> GKAFDDGAFTGIREINLSYNKETAIGDFQVVYDLNGSPYVGENHKSFITGFTPVKISLDFPSEYIMEVSGYTGKVSGYVVVRSLTFKTNKKTYGPYGVTSGTPFSLPIENGLIVGFKGSIGYWL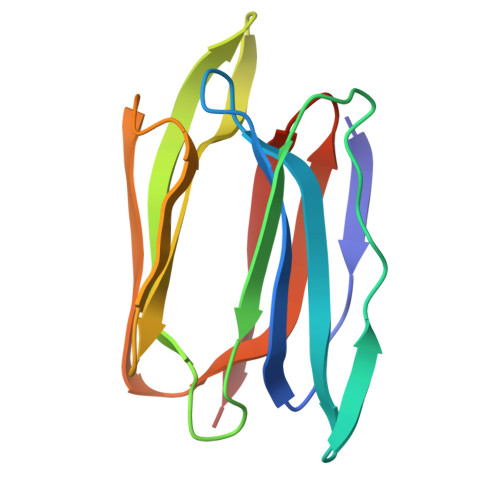DYFSMYLSL ORTHO-XYLENE | C8 H10 | 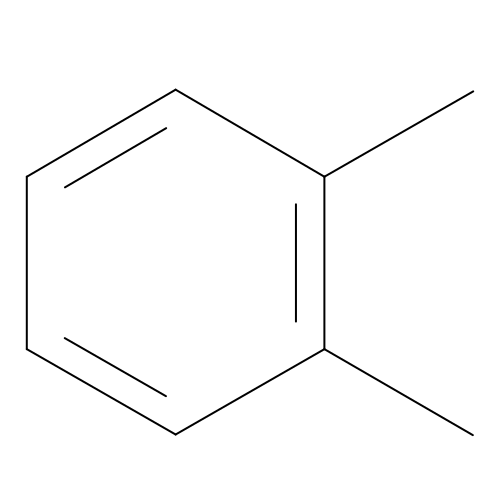CTQNGGLPUBDAKN-UHFFFAOYSA-N2-Phenylacrylic acid | C9 H8 O2 | 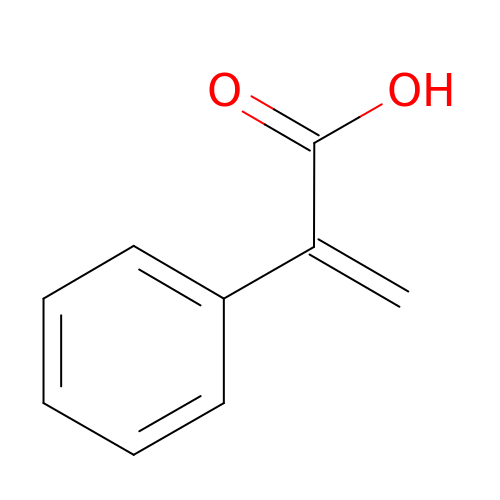ONPJWQSDZCGSQM-UHFFFAOYSA-N Aminoacyl-tRNA synthetases (AARSs), a family of essential protein synthesis enzymes, are attractive targets for drug development. Here we present five unusual crystal structures showing that threonyl-tRNA synthetase (ThrRS) is covalently inhibited by a natural product, obafluorin (OB). OB contains a β-lactone ring with a 2,3-dihydroxybenzamidyl moiety attached to the α position and a 4-nitrobenzyl moiety attached to the β position. When ThrRS catalyzes tRNA aminoacylation, the Zn2+ ion recognizes and binds l-threonine, assisting in the l-threonine activation reaction.

To elucidate the mechanism by which OB inhibits ThrRS, we cocrystallized a fragment of Escherichia coli ThrRS containing catalytic and anticodon-binding domains (residues 242–642) with OB and determined the structure to a resolution of 2.5 Å. In the two catalytic domains of ThrRS homodimer, OB was bound to the active site for Thr-AMP formation. In total, 18 residues in the active center of ThrRS were located within 4.5 Å of OB and thus interacted with it. Interestingly, the four-membered ring of the β-lactone of OB was opened in the ThrRS-OB structure. Instead, the acyl group formed a new ester bond with the phenolic group of Tyr462. In addition, the two hydroxyl groups on the o-diphenol moiety of OB formed two coordination bonds with the conserved catalytic Zn2+ ion of ThrRS. This structure suggests that OB inhibits ThrRS by forming coordination bonds with the Zn2+ ion in the catalytic center of ThrRS, allowing its β-lactone ring to be approached and attacked by the phenolic group of Tyr462, and finally forming a new covalent bond with Tyr462. The ThrRS-OB structure showed that the o-diphenol group of OB occupied the position of l-threonine and replaced it to bind Zn2+ ion and Asp383. At the same time, the conformations of Gln484 and Met332 were changed to accommodate OB. Therefore, the nitrobenzene group of OB occupied the binding site of tRNA A76, which prevented tRNA from entering the active center of ThrRS.

>MRDHRKIGKQLDLYHMQEEAPGMVFWHNDGWTIFRELEVFVRSKLKEYQYQEVKGPFMMDRVLWEKTGHWDNYKDAMFTTSSENREYCIKPMNCPGHVQIFNQGLKSYRDLPLRMAEFGSCHRNEPSGSLHGLMRVRGFTQDDAHIFCTEEQIRDEVNGCIRLVYDMYSTFGFEKIVVKLSTRPEKRIGSDEMWDRAEADLAVALEENNIPFEYQLGEGAFYGPKIEFTLYDCLDRAWQCGTVQLDFSLPSRLSASYVGEDNERKVPVMIHRAILGSMERFIGILTEEFAGFFPTWLAPVQVVIMNITDSQSEYVNELTQKLSNAGIRVKADLRNEKIGFKIREHTLRRVPYMLVCGDKEVESGKVAVRTRRGKDLGSMDVNEVIEKLQQEIRSRSLKQLEELEHHHHHH[2x]> NALICEDKSCFWKKNANNIVEVPYVVSGEFSINDKSVIANAISIFHAQTCIRFVPRSIQADYLSIENKDGCYSAIGRT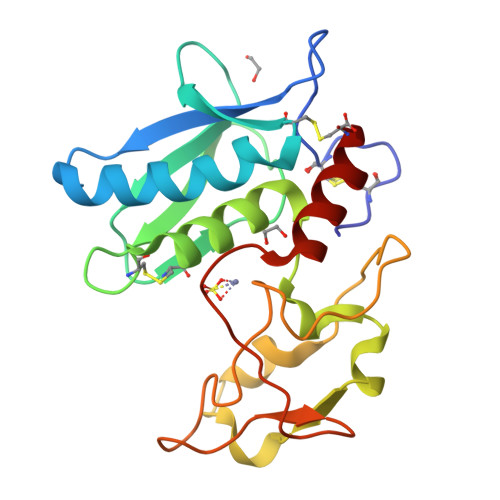GGKQVVSLNRKGCVYSGIAQHELNHALGFYHEQSRSDRDQYVRINWNNISPGMAYNFLKQKTNNQNTPYDYGSLMHYGKTAFAIQPGLETITPIPDENVQIGQRQGLSKIDILRINKLYGC>QSVDIHKDQIIFSEGDAGDCAYIIEKGRVLIYLTKDKEEIPLTILGEGEIFGEMALIDNQNRSASVRALEDVRLAIVTKQQVLERVSTADKVVQLLMRVLLKRLRRKNIGGPGGSRISEVEFDNSGAGDDGTQSALDQIKLENQIFQAFQNKEFELFYQPIVNLKNKTITGCEALLRWNSPQHGLVSPNLFIDIIENSSMVIPIGHWIINQALKDLRTIQDQLRLNKKERMADDFMMSINISGRQFTHSDFVNNLEDLREKHDLHTQNIKLEMTERIMMDGAIAIDALNQCRSLGYAISIDDFGTGFSGLQYLTQMPISFLKIDRSFVMKILSDPKSKAVVSSIIHLAHAMDIEVIAEGIEHHEEALVLETLGARFGQ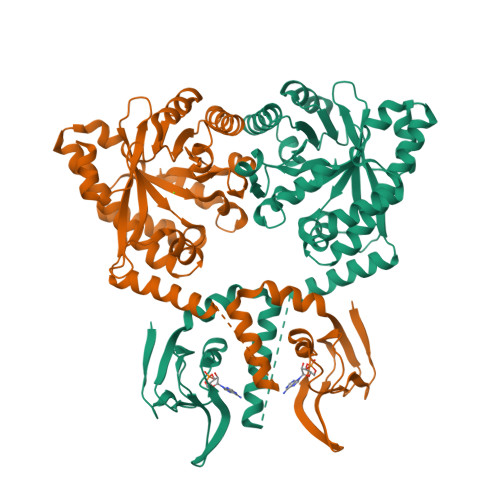GYLFSKPVDLGRFLKLIKL[2x]>MLPRLICINDYEQHAKSVLPKSIYDYYRSGANDEETLADNIAAFSRWKLYPRMLRNVAETDLSTSVLGQRVSMPICVGATAMQRMAHVDGELATVRACQSLGTGMMLSSWATSSIEEVAEAGPEALRWLQLYIYKDREVTKKLVRQAEKMGYKAIFVTVDTPYLGNRLDDVRNRFKLPPQLRMKNFETSTLSFSPEENFGDDSGLAAYVAKAIDPSISWEDIKWLRRLTSLPIVAKGILRGDDAREAVKHGLNGILVSNHGARQLDGVPATIDVLPEIVEAVEGKVEVF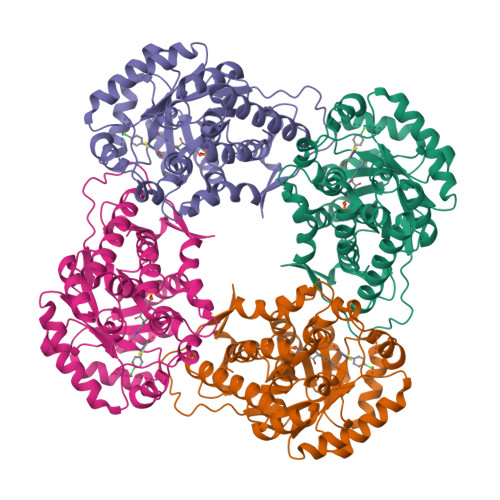LDGGVRKGTDVLKALALGAKAVFVGRPIVWGLAFQGEKGVQDVLEILKEEFRLAMALSGCQNVKVIDKTLVRKNPLAVSKI[4x]>[2x]SNSITENTSWNKEFSAEAVNGVFVLCKSSSKSCATNDLARASKEYLPASTFKIPNAIIGLETGVIKNEHQVFKWDGKPRAMKQWERDLTLRGAIQVSAVPVFQQIAREVGEVRMQKYLKKFSYGNQNISGGIDKSWLEDQLRISAVNQVEFLESLYLNKLSASKENQLIVKEALVTEAAPEYLVHSKTGFSGVGTESNPGVAWWVGWVEKETEVYFFAFNMDIDNESKLPLRKSIPTKIMESEGIIGG

OXA-10 (PSE-2) is a class D β-lactamase that was originally described in the late 1970s and confers resistance to cefotaxime and ceftriaxone but not to ceftazidime. Natural and laboratory-selected variants of OXA-10 have been identified, many of which differ in the spectrum of β-lactams that they hydrolyze. Class D β-lactamases share the same general structure with conserved motifs, including an active-site serine 67, a carbamylated lysine (K70), and a stabilizing and invariant tryptophan residue (W154) within the Ω-loop. We were able to determine apo structures for both enzymes but not in complex with ceftazidime. Both protein structures contained two chains in the asymmetric unit, corresponding to a dimer, as previously described for OXA-10 (14, 24).

OXA-935 differs from OXA-10 by two amino acid substitutions: G157D, which it shares with OXA-14, and F153S which is novel. OXA-935 differs from OXA-14 in a single amino acid substitution in the protein’s Ω-loop at position 153. The amino acid change F153S introduced high flexibility into the Ω-loop of OXA-935. In contrast, the Ω-loops of both chains in the crystal structure of OXA-935 had open conformations where the hydrogen bond between K70 and the indole group of W154 was absent (16.4 Å) and both of the K70 residues were decarbamylated. This more open confirmation of the Ω-loop created a larger and more positively charged active site cavity, which may allow it to accommodate bulkier and more negatively charged substrates, such as ceftazidime. The F153S variant found within OXA-935 yielded a distinctly different structure of the Ω-loop, in which W154 was considerably more flexible and oriented away from the active site cavity, the carbamylation of K70 was not observed, and the active site groove was more positively charged. The carbamylation of K70 in other class D β-lactamases is favored at a more basic pH, whereas OXA-935 showed decarbamylated K70 even at a pH of 8.3. Thus, unlike OXA-10, OXA-14, and other related β-lactamases, it is likely that the K70 of OXA-935 remains decarbamylated in vitro, despite increases in pH. In contrast, OXA-935 showed higher affinity (Km = 17 μM) and substrate turnover (kcat = 0.24 s−1) for ceftazidime than did OXA-14. Therefore, OXA-935, despite having a more flexible Ω-loop and decarbamylated K70, hydrolyzed ceftazidime more efficiently in vitro than did OXA-14, consistent with the observed ceftazidime resistance phenotype in our P. aeruginosa isolates.>DAKAATKLADGKYNIAFTVWKGDKDESSRMNRYFESPATLTVKNGKQYVSFKVKDSTSIKSFQVEKDGQFVETTVLSEN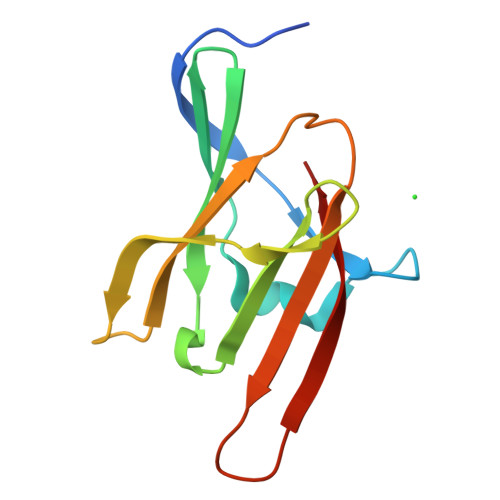KKDNTRVVEFEVADLSKKLNGKVKINIPIINYNASYDIRFVF[2x]>[2x]SNAYRQSQSRAARLRLLVDTGQELIQLPPEAMRKCVLQRACAFVAMDHGLLLEWGA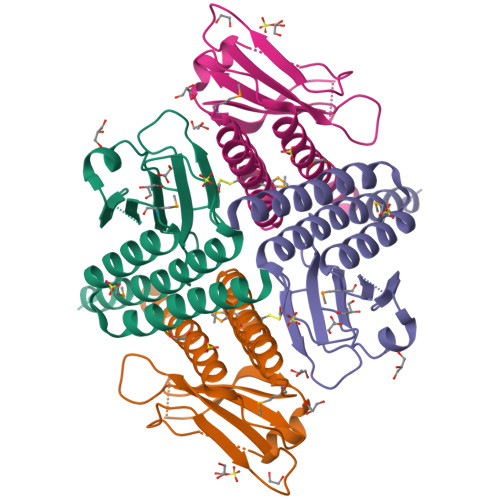DNGVQTTARHGSKERLSTLETTADPLAIGPQWLERPGTHLPCVLLLPLRGADEGSFGTLVLANSVAISAPDGEDIESLQLLATLLAAHLENNRLLEALVARDRT> MAKGKSEVVEQNHTLILGWSDKLGSLLNQLAIANESLGGGTIAVMAERDKEDMELDIGKMEFDFKGTSVICRSGSPLILADLKKVSVSKARTI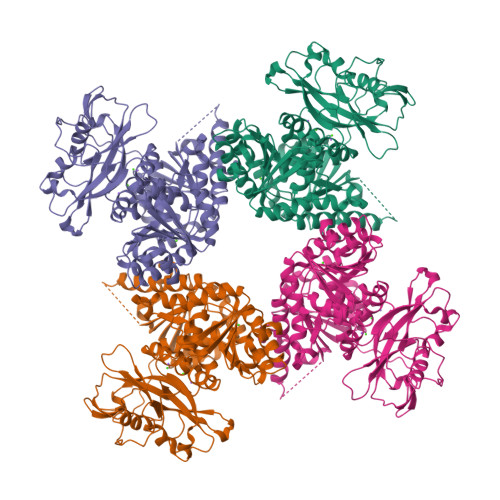IVLAEDGNADQSDARALRTVLSLTGVKEGLRGHIVVEMSDLDNEVLVKLVGGDLVETVVAHDVIGRLMIQCARQPGLAQIWEDILGFENCEFYIKRWPQLDGMLFEDVLISFPAAIPCGIKVASYGGKIILNPDDSYVLQEGDEVLVIAEDDDTYAPAPLPMVRRGSLPKDFVYPKSPERILFCGWRRDMEDMITVLDASLAPDSELWMFNDVPEKEREKKLIDGGLDISRLENISLVNREGNAVIRRHLESLPLESFDSILILADESVEDSAIQADSRSLATLLLIRDIQARRLPYVAMASQTQGGNFSKGSWIGEMKQASDKTVIISEILDPRTKNLLSMSKISDYVLSNELVSMALAMVAEDRQINDVLEELFAEEGNEMHIRQADIYLREGEEMSFYEIMLRARQRREILIGYRLANAERAVINPPAKTGRRKWSLKDVFVVITEKEGSRSHHHHHH>MGKSLSHLPLHSSKEDAYDGVTSENMRNGLVNSEVHNEDGRNGDVSQFPYVEFTGRDSVTCPTCQGTGRIPRGQENQLVALIPYSDQRLRPRRTKLYVMASVFVCLLLSGLAVFFLFPRSIDVKYIGVKSAYVSYDVQKRTIYLNITNTLNITNNNYYSVEVENITAQVQFSKTVIGKARLNNISIIGPLDMKQIDYTVPTVIAEEMSYMYDFCTLISIKVHNIVLMMQVTVTTTYFGHSEQISQERYQYVDCGRNTTYQLGQSEYLNVLQPQQ[8x]

pmcAmyotrophic lateral sclerosis/parkinsonism-dementia complex (ALS/PDC or lytico-bodig) is a fatal disease found in the Chamorro population of Guam (1–4), some families on the Kii peninsula of Japan, and the Auyu and Jakai people of New Guinea. Abundant filamentous amyloid inclusions that are made of all six brain tau isoforms are characteristic of ALS/PDC. We now show that tau filaments from Guam and Kii ALS/PDC adopt the CTE fold in brain and spinal cord. The greater heterogeneity of amyloid filaments, when compared to CTE and SSPE, probably reflects the fact that ALS/PDC is a multiple proteinopathy based on neuropathology, as suggested for cases from the Kii peninsula.

In addition to tau filaments, we also observed singlets and doublets of transmembrane protein 106B (TMEM106B) filaments (fold I) in the frontal cortex from cases 1 and 2, and TMEM106B singlets (fold I) in the spinal cord from case 2. Senile plaques have been described in around 60% of cases of Guam ALS/PDC and assembly of Aβ is believed to be part of the disease process. Alternatively, these changes may be age-related. This was probably also the reason for the presence of TMEM106B filaments in two cases from Guam and one case from the Kii peninsula.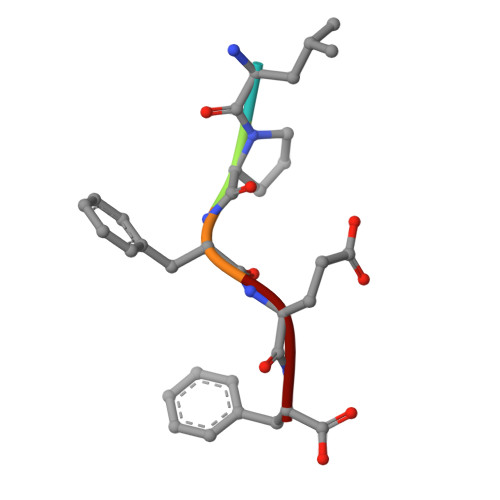> LPFEF> MQKRVTDEEIKERLGKIKSRIAVMSGKGGVGKSTVTALLAVHYARQGKKVGILDADFLGPSIPIL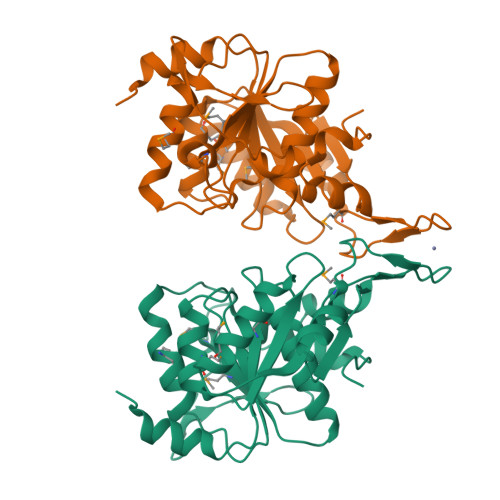FGLRNARIAVSAEGLEPVLTQKYGIKVMSMQFLLPKENTPVIWRGPLIAGMIREFLGRVAWGELDHLLIDLPPGTGDAPLTVMQDAKPTGVVVVSTPQELTAVIVEKAINMAEETNTSVLGLVENMSYFVCPNCGHKSYIFGEGKGESLAKKYNIGFFTSIPIEEELIKLADSGRIEEYEKDWFESAPFLEHHHHHH>[3x]MSEIVKFNPVMASGFGAYIDHRDFLEAKTETIKNLLMRQGFVVVKNLDIDSDTFRDIYSAYGTIVEYADEKIGVGFGYRDTLKLEGEKGKIVTGRGQLPFHADGGLLLSQVDQVFL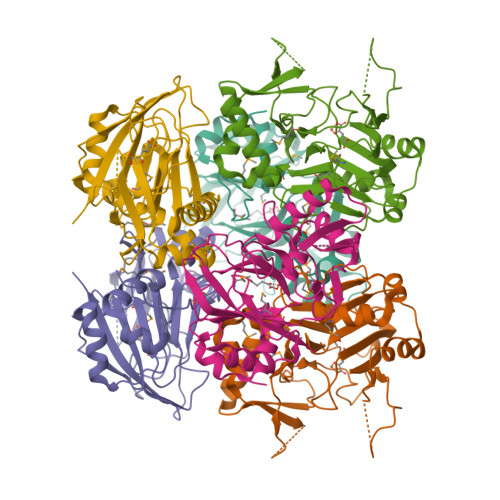YAAEIKNVKFRGATTVCDHALACQEMPAHLLRVLEEETFEVRVLERGYYVDVSPDGWFKVPVFTDLGWVRKMLIYFPFDEGQPASWEPRIVGFTDHETQAFFQELGAFLKQPRYYYKHFWEDGDLLIMDNRRVIHEREEFNDDDIVRRLYRGQTADI> AECSVDIQGNDQMQFNTNAITVDKSCKQFTVNLSHPGNLPKNVMGHNWVLSTAADMQGVVTDGMASGLDKDYLKPDDSRV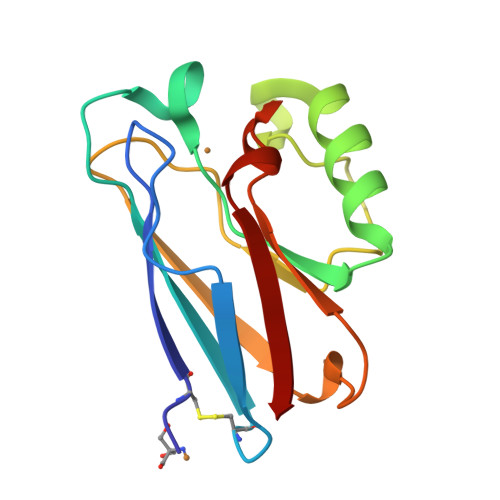IAHTKLIGSGEKDSVTFDVSKLKEGEQYMFFDTFPGHSALFKGTLTLK>MIDCAIIGGGPAGLSAGLYATRGGVKNAVLFEKGMPGGQITGSSEIENYPGVKEVVSGLDFMQPWQEQCFRFGLKHEMTAVQRVSKKDSHFVILAEDGKTFEAKSVIIATGGSPKRTGIKGESEYWGKGVSTCATCDGFFYKNKEVAVLGGGDTAVEEAIYLANICKKVYLIHRRD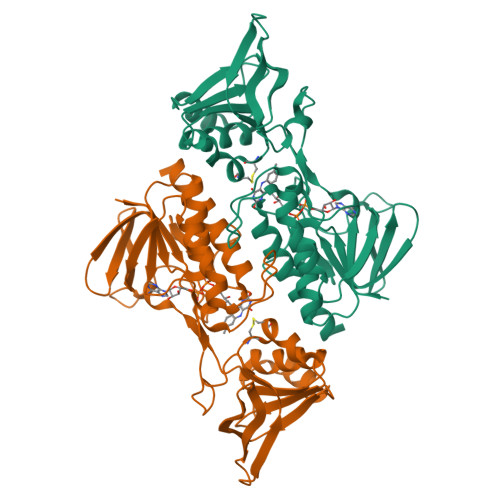GFRCAPITLEHAKNNDKIEFLTPYVVEEIKGDASGVSSLSIKNTATNEKRELVVPGFFIFVGYDVNNAVLKQEDNSMLCKCDEYGSIVVDFSMKTNVQGLFAAGDIRIFAPKQVVCAASDGATAALSVISYLEHH[3x]>[2x]CCACUGAGAGCUUC;>GGAAGCUCUGACCGACCCCCAGCC[2x];>[2x]GCUGGG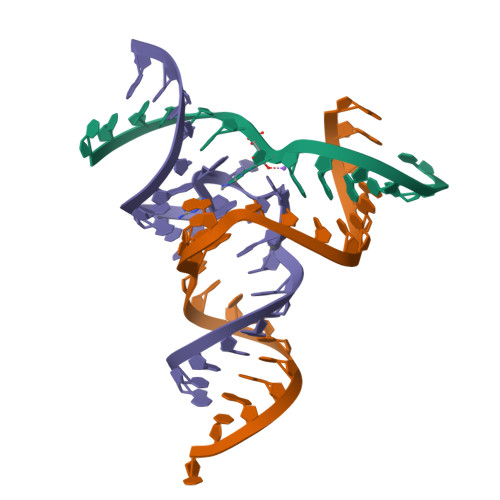ACAACUAGACAUACAGUG>GSHMKDQMETSYVSLKTWIEDSLDLFKNDLLPLLYPLFIHIYFDLIQQNKTDEAKEFFEKYRGDHYNKSEEIKQFESIYTVQHIHENNFAYTFKNSKYHLSMGRYAFDLLIN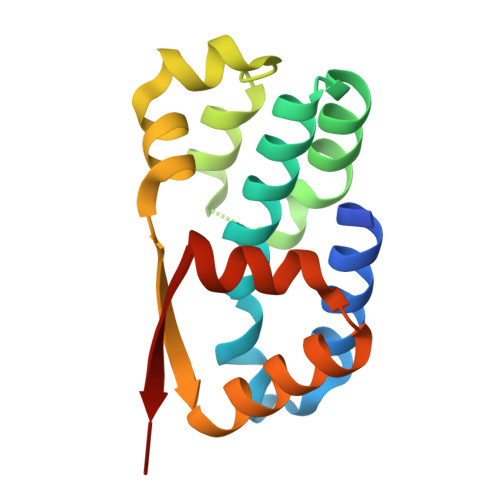FLEERNLTYILKILNQHLDIKVYVGP[5x]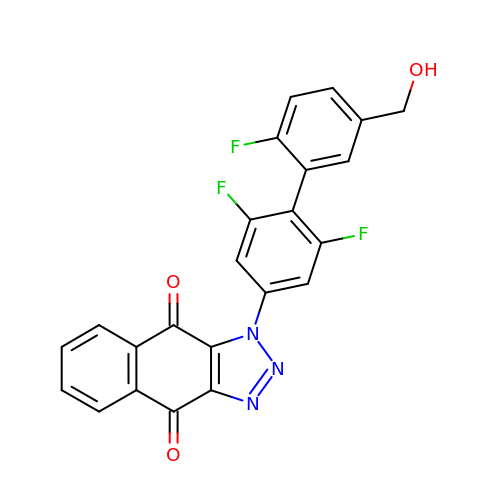3-[3,5-bis(fluoranyl)-4-[2-fluoranyl-5-(hydroxymethyl)phenyl]phenyl]benzo[f]benzotriazole-4,9-dione | C23 H12 F3 N3 O3 | JWRMSFLQXIFPOJ-UHFFFAOYSA-N>GSMKKEFTELYDFIFDPIFLVRYGYYDRSIKNKKMNTAKVELDNEYGKSDSFYFKVFNMESFADYLRSHDLKTHFNGKKPLSTDPVYFNIPKNIEARRQYKMPNLYSYMALNYYICDNKKEFIEVFIDNKFSTSKFFNQLNFDYPKTQEITQTLLYGGIKKLHLDLSNFYHTLYTHSIPWMIDGKSASKQNRKKGFSNTLDTLITACQYDETHGIPTGNLLSRIITELYMCHFDKQMEYKKFVYSRYVDDFIFPFTFENEKQEFLNEFNLICRENNLIINDNKTKVDNFPFVDKSSKSDIFSFFENITSTNSNDKWIKEISNFIDYCVNEEHLGNKGAIKCIFPVITNTLKQKKVDTKNIDNIFSKRNMVTNFNVFEKILDLSLKDSRLTNKFLTFFENINEFGFSSLSASNIVKKYFSNNSKGLKEKIDHYRKNNFNQELYQILLYMVVFEIDDLLNQEELLNLIDLNIDDYSLILGTILYLKNSSYKLEKLLKKIDQLFINTHANYDVKTSRMAEKLWLFRYFFYFLNCKNIFSQKEINSYCQSQNYNSGQNGYQTELNWNYIKGQGKDLRANNFFNELIVKEVWLISCGENEDFKYLN[6x]

Abortive infection (Abi) is a bacterial antiphage defense strategy involving suicide of the infected cell. Some Abi pathways involve polymerases that are related to reverse transcriptases. They are unique in the way they combine the ability to synthesize DNA in a template-independent manner with protein priming. Here, we report crystal and cryo-electron microscopy structures of two Abi polymerases: AbiK and Abi-P2. Both proteins adopt a bilobal structure with an RT-like domain that comprises palm and fingers subdomains and a unique helical domain.

We also obtained crystals of Ll-AbiK that diffracted X-rays to 3.1 Å resolution. The polypeptide chain was first traced into the cryo-EM maps, and the resulting model was used to solve the crystal structure by molecular replacement. In the crystal structure of Ll-AbiK, eight to ten nucleotides of the DNA chain could be defined for individual protomers. In all subunits, the DNA’s 5′ end is covalently attached to the hydroxyl group of Tyr44, which for the first time demonstrates that this tyrosine serves to prime DNA synthesis in Ll-AbiK. Tyr44 is located in the middle of a long loop (residues 21–57) that essentially lacks secondary structure elements. In the wild-type Ll-AbiK–DNA adduct crystal structure, downstream from the first nucleotide that is attached to the tyrosine residue, the DNA strand makes a turn and continues through the channel between the polymerase and helical domain toward the active site, which is formed by Asp163, Asp247 and Asp248 and is located close to the center of the hexamer. In this channel, nucleotides −2, −3 and −4 (numbering in 5′-3′ direction with nt −1 located near the active site) are stabilized by stacking interactions between nucleobases and aromatic side chains that line the sides of the channel (Tyr142, Tyr245 and Phe299). Interactions are also formed with the phosphate backbone (mediated by Asp141) and with nucleobases (mediated by Tyr145, Lys295, and Asn346). In the crystallographic data a continuous electron density for the entire DNA chain is only observed in one of the subunits of the hexamer. For the other protomers, the electron density contains a gap after the second nucleotide.> MDASTLFKKVKVKRVLGSLEQQIDDITTDSRTAREGSIFVASVGYTVDSHKFCQNVADQGCKLVVVNKEQSLPANVTQVVVPDTLRVASILAHTLYDYPSHQLVTFGVTGTNGKTSIATMIHLIQRKLQKNSAYLGTNGFQINETKTKGANTTPETVSLTKKIKEAVDAGAESMTLEVSSHGLVLGRLRGVEFDVAIFSNLTQDHLDFHGTMEAYGHAKSLLFSQLGEDLSKEKYVVLNNDDSFSEYLRTVTPYEVFSYGIDEEAQFMAKNIQESLQGVSFDFVTPFGTYPVKSPYVGKFNISNIMAAMIAVWSKGTSLETIIKAVENLEPVEGRLEVLDPSLPIDLIIDYAHTADGMNKLIDAVQPFVKQKLIFLVGMAGERDLTKTPEMGRVACRADYVIFTPDNPANDDPKMLTAELAKGATHQNYIEFDDRAEGIKHAIDIAEPGDTVVLASKGREPYQIMPGHIKVPHRD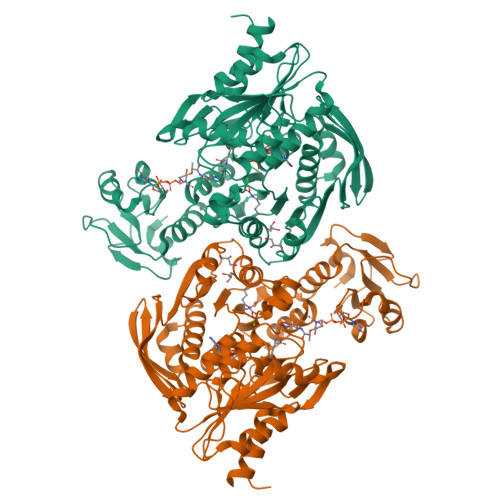DLIGLEAAYKKFGGGPVDRSHHHHHH>[2x]GSPNSGTASNGSTQQLPQTIIIGVRKGGTRALLEMLSLHPDVAAAENEVHFFDWEEHYSQGLGWYLTQMPFSSPHQLTVEKTPAYFTSPKVPERIHSMNPTIRLLLILRDPSERVLSDYTQVLYNHLQKHKPYPPIEDLLMRDGRLNLDYKALNRSLYHAHMLNWLRFFPLGHIHIVDGDRLIRDPFPEIQKVERFLKLSPQIN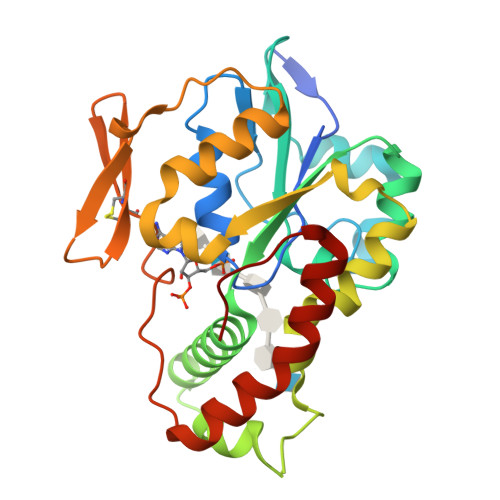ASNFYFNKTKGFYCLRDSGKDRCLHESKGRAHPQVDPKLLDKLHEYFHEPNKKFFKLVGRTFDWH>GPHMTGLAAISDALAADLAGLSFSSPVAHVYNPLLYAREPHVAYLSRFGSPPKEVLFVGMNPGPWPMAQTGVPFGEVAVVTEWLGINGTVTRPAGEHPKKRVDGFACRRSEVSGRRLWGFIRERFGTPERFFARFFVANYCPLLFLTAEGGNITPDKLRRGEQEPLFAACDLALRRTVVLLRPRVVIGVGAFAEARCHEALEGFDVEV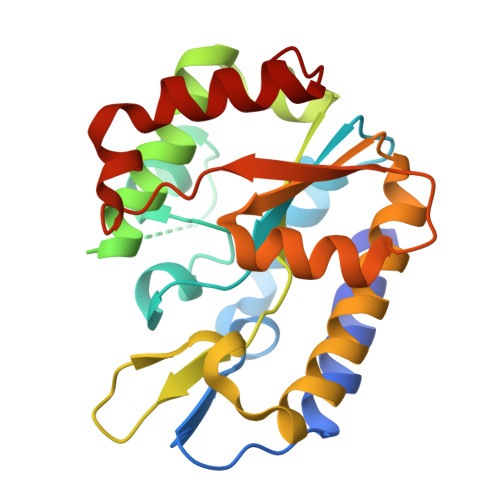GRIIHPSPASPAANRDWAGTALRQLAELGVDF[2x]>MSDKYYRSAYMNVDLNAVASNFKVFSTLHPNKTVMAVVKANAYGLGSVKVARHLMENGATFFAVATLDEAIELRMHGITAKILVLGVLPAKDIDKAIQHRVALTVPSKQWLKEAIKNISGEQEKKLWLHIKLDTGMGRLGIKDTNTYQEVIEIIQQYEQLVFEGVFTHFACADEPGDMTTEQYQRFKDMVNEAIKPEYIHCQNSAGSLLMDCQFCNAIRPGISLYGYYPSEYVQQKVK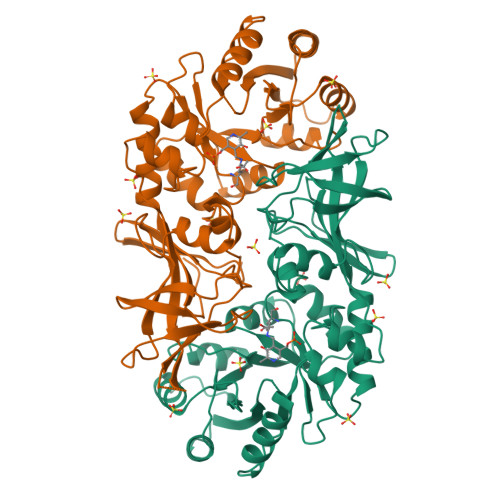VHLKPSVQLIANVVQTKTLQAGESVSYGATYTATDPTTIALLPIGYADGYLRIMQGSFVNVNGHQCEVIGRVCMDQTIVKVPDQVKAGDSVILIDNHRESPQSVEVVAEKQHTINYEVLCNLSRRLPRIYHDGDQRFVTNELLK[2x]> MLAEKTRSIIKATVPVLEQQGTVITRTFYKNMLTEHTELLNIFNRTNQKVGAQPNALATTVLAAAKNIDDLSVLMDHVKQIGHKHRALQIKPEHYPIVGEYLLKAIKEVLGDAATPEIINAWGEAYQAIADIFITVEKKMYEEALWPGWKPFEITAKEYVASDIVEFTVKPKFGSGIELESLPITPGQYITVNTHPIRQENQYDALRHYSLCSASTKNGLRFAVKMEAARENFPAGLVSEYLHKDAKVGDEIKLSAPAGDFAINKELIHQNEVPLVLLSSGVGVTPLLAMLEEQVKCNPNRPIYWIQSSYDEKTQAFKKHVDELLAECANVDKII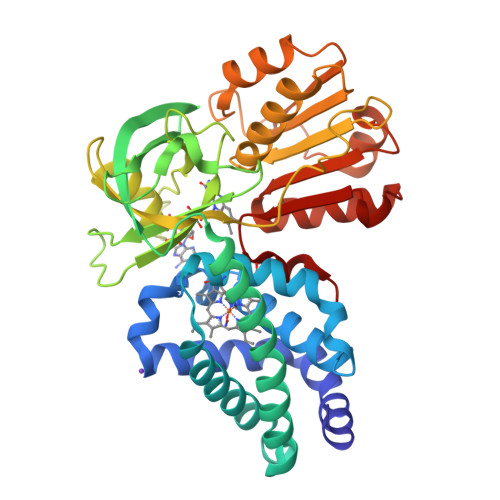VHTDTEPLINAAFLKEKSPAHADVYTCGSLAFMQAMIGHLKELEHRDDMIHYEPFGPKMSTVQV The sulfonamides (sulfas) are the oldest class of antibacterial drugs and inhibit the bacterial dihydropteroate synthase (DHPS, encoded by folP), through chemical mimicry of its co-substrate p-aminobenzoic acid (pABA). Resistance to sulfa drugs is mediated either by mutations in folP or acquisition of sul genes, which code for sulfa-insensitive, divergent DHPS enzymes. DHPS catalyzes the condensation of para-aminobenzoic acid (pABA) and 6-hydroxymethyl-7,8-dihydropterin pyrophosphate (DHPP), producing 7,8-dihydropteroic acid (7,8-DHP); this compound is further transformed, ultimately leading to tetrahydrofolate, an essential precursor for DNA and RNA synthesis. All three Sul enzymes adopted the (ɑ/β)8 TIM barrel fold also shared by DHPS.

We determined the crystal structure of Sul1 in a ligand-bound state, and the Sul2 and Sul3 enzymes in both apo and ligand-bound forms to resolutions between 1.74 to 2.8 Å. Comparison of Sul apo and ligand-bound structures revealed conformational changes in these three loops triggered by ligand binding. In particular, loop 1 is oriented further away from the ligand-binding cleft in the apo structures of Sul2 and Sul3 as compared to the structures of these enzymes in 7,8-DHP or pABA-bound states. Similarly, loop 3 in Sul2 and Sul3 also undergoes a large conformational change upon binding of pABA or 7,8-DHP. Finally, in the Sul2 and Sul3 structures, loop 2 undergoes conformational changes in a more confined space in presence of the ligands. We noticed that the Phe residue that is conserved across Sul enzymes (Phe178 in Sul1, Phe179 in Sul2 and Phe177 in Sul3) and localized to the active site adopted different rotamer conformations depending on ligand binding.

>[4x]QGMSKIFGIVNITTDSFSDGGLYLDTDKAIEHALHLVEDGADVIDLGAASSNPDTTEVGVVEEIKRLKPVIKALKEKGISISVDTFKPEVQSFCIAAAVDFINDIQGFPYPEIYSGLAKSDCKLVLMHSVQRIGAATKVETNPEEVFTSMMEFFKERIAALVEAGVKRERIILDPGMGFFLGSNPETSILVLKRFPEIQEAFNLQVMIAVSRKSFLGKITGTDVKSRLAPTLAAEMYAYKKGADYLRTHDVKSLSDALKISKALG>MRVLVTRTLPGKALDRLRERGLEVEVHRGLFLPKAELLKRVEGAVGLIPTVEDRIDAEVMDRAKGLKVIACYSVGVDHVDLEAARERGIRVTHTPGVLTEATADLTLALLLAVARRVVEGAAYARDGLWKAWHPELLLGLDLQGLTLGLVGMGRIGQAVAKRALAFGMRVVYHARTPKPLPYPFLSLEELLKEADVVSLHTPLTPETHRLLNRERLFAMKRGAILLNTARGALVDTEAL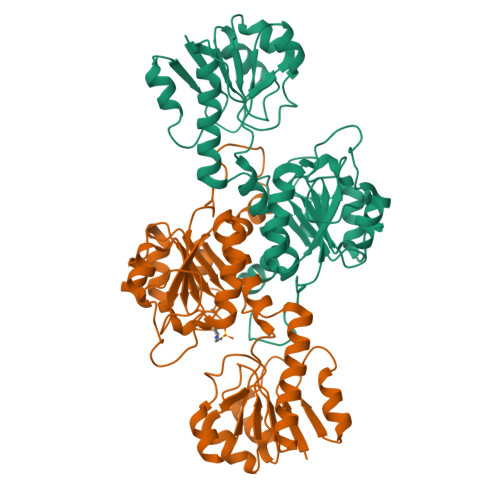VEALRGHLFGAGLDVTDPEPLPPGHPLYALPNAVITPHIGSAGRTTRERMAEVAVENLLAVLEGREPPNPVV[4x]> ACDYTCGSNCYSSSDVSTAQAAGYKLHEDGETVGSNSYPHKYNNYEGFDFSVSS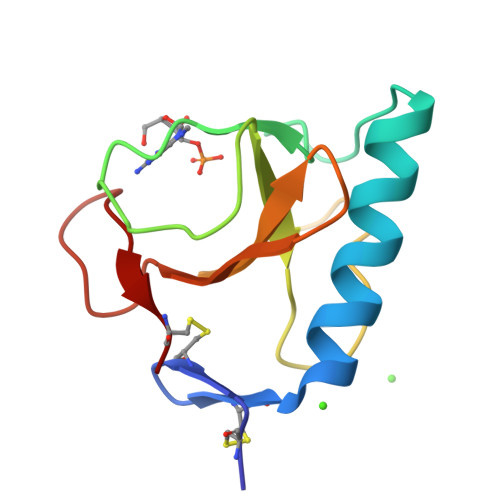PYYEWPILSSGDVYSGGSPGADRAVFNENNQLAGVITHTGASGNNFVECT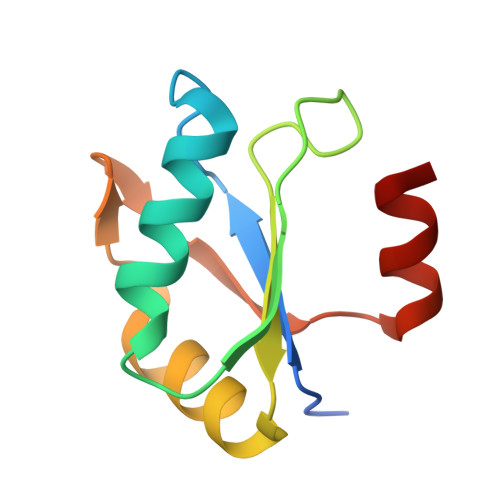> GAMEMLPNQTIYINNLNEKIKKEELKKSLYAIFSQFGQILDIVALKTLKMRGQAFVIFKEIGSASNALRTMQGFPFYDKPMQIAYSKSDSDIVAKIKG>RPMDNEAVQFGMSMGIGWNLGNQMDAHYDGCSYETGWGNKAATQQTFNGLAKAGFRSVRIPVTWMGHIGNAPTYAIERGWLDRVDELVHMAHKAGLIVIINIHHDGFGAADTPSKGSHWLDLPAAVASEERNQLIKQELTMIWLQIGKRFANDGEWLVFETLNAIQDGDWGNGNNRRDGGAQYRVLNEWNQVCVDAIRAAGGKNETRYIGVPGYVCNPDLTVENLVLPEDVVPNRLMVAVHSYDPWDYAGSAKYNEWGHTGKDVVPGVGEEAYVGMLNRLFNMYIRRGVPVYFGEFGAVRRASKADEEFRLYYFRYICKAMRDRRISALYWDNGNSKAGNDGFGVIDHATGRFIGNGEQAVRAMIDSWENNDPNYTLQSIYDSAPESSR[2x]

AC2aCel5A is an endo-acting cellulase that is encoded within the first reported cellulolytic PUL, originating from an uncultured Bacteroidetes phylotype. As previously reported, AC2aCel5A is an endoglucanase active on β-(1,4) glycosidic bonds between glucose units in soluble and insoluble cellulosic substrates and in linear β-glucans. The enzyme displays the typical (β/α)8 barrel structure associated with the GH5 family. The six closest structural homologues, which include all the biochemically characterized members of subfamily GH5_4, were identified using the Dali server17 and were used to produce a structure-based multiple sequence alignment using the PROMALS3D server. This allowed identification of the conserved catalytic residues, i.e. Glu172 and Glu303, acting as the catalytic acid and nucleophile/base, respectively.

The roles of Glu172 and Glu303 as catalytic residues were confirmed by site-directed mutagenesis experiments, showing that AC2aCel5A_EE172A and AC2aCel5A_EE303A were both inactive in the standard carboxymethylcellulose (CMC) assay. Co-crystallization of the E172A mutant with cellotetraose resulted in the complex structure solved to 2.4 Å resolution, with two molecules in the asymmetric unit. Additional electron density was observed in the active-site cleft of molecule A, and was refined as a cellotriose molecule bound to the −3 to −1 subsites. No electron-density for a bound ligand could be observed in the B molecule, which also lacked electron density for several main-chain residues, namely 34–45 and 112–127. Even though the ligand density appears to fit a cellotriose molecule, it is likely that a cellotetraose molecule is present in the complex as the enzyme only produces dimers from cellotetraose. The observed cellotriose density could reflect three glucose moieties of a tetramer, where the fourth moiety could be positioned in the putative −4 position and be disordered. The glucose moiety bound in the −1 subsite is stabilized by hydrogen bonding from its O2 group to the catalytic Glu303 residue, as well as the strictly conserved Asn171. Unlike the sugars bound in the −2 and −1 subsites, the sugar bound in the −3 subsite involves no hydrogen bonds between the ligand and the protein. Its binding seems to be mediated by stacking interactions with Trp45. Superposition of the native structure on the cellotriose complex placed a carboxyl oxygen of the catalytic acid, Glu172, at 1.7 Å of O1 of the glucose bound in the −1 subsite.> MIRTTNTCCGNQAG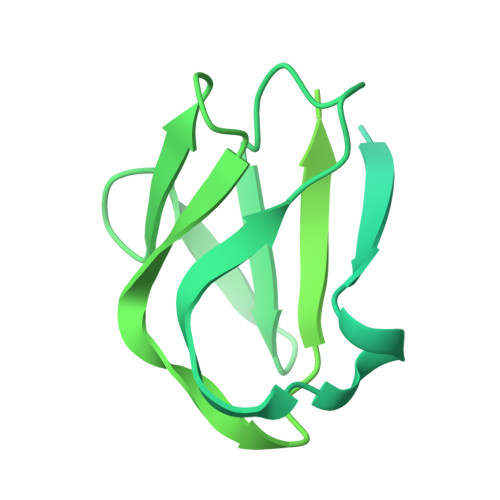MVEKFIGTAYDVVKTVYDNLGEIQFIYNFLNDYGVLITVDSVTELQELPTTAKYTRVYSSTPTGVRIYTDYLYVEGDRTGVLPSDPTATGSWVVVGSSNSGAATGTGAYIPFVFNNGSAAGGETTIVVPDYTIGVPEIYVEGFRQQVGRGFTFNSVNLTVTLAQPLEQGDEVVLMLSGNPAVPDNPNIDSWTVINWIYNNGAAVGGEQVIVIPYTFQTVPAIFKNGLRYQGGLSTQSYTVDQDNKRILLTEPLSTNDRLVVQLGGELVTLESPDRSLYEIARATNMKDSEVIKSDNTVETLNGKRILYDIVSQVYYWIPSSVPNNVYIQSVVNGQLTYLPGNIVVTLTPIVTLGLSGTTAQRPIGVLTGTQHFDTTLGKPIWFNGTAWVDSTGAVV> QFAKPEDAVKYRQ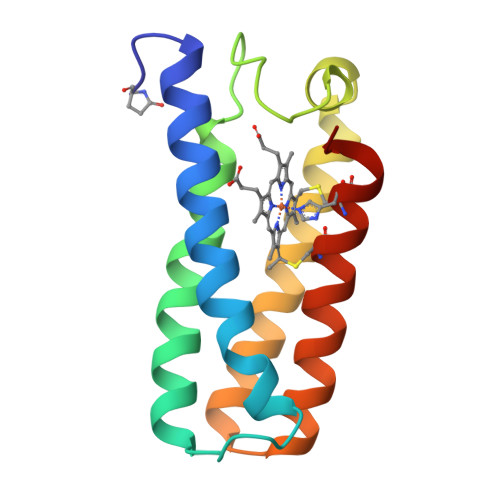SALTLMASHFGRMTPVVKGQAPYDAAQIKANVEVLKTLTALPWAAFGPGTEGGDARPEIWSDAASFKQKQQAFQDNIVKLSAAADAGDLDKLRAAFGDVGASCKACHDAYRKKK2-[4-(4-cyano-3-methylphenoxy)phenyl]-N-methyl-N-[2-(5-methyl-1,2,4-oxadiazol-3-yl)ethyl]acetamide | C22 H22 N4 O3 | 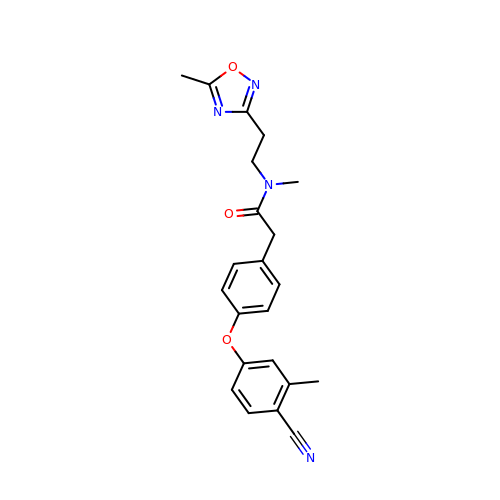IRHPSNSMVQKDNH-UHFFFAOYSA-N>[2x]MPINRPNLNLNIPPLNIVAAYDGAEIPSTNKHLKNNFNSLHNQMRKMPVSHFKEALDVPDYSGMRQSGFFAMSQGFQLNNHGYDVFIHARRESPQSQGKFAGDKFHISVLRDMV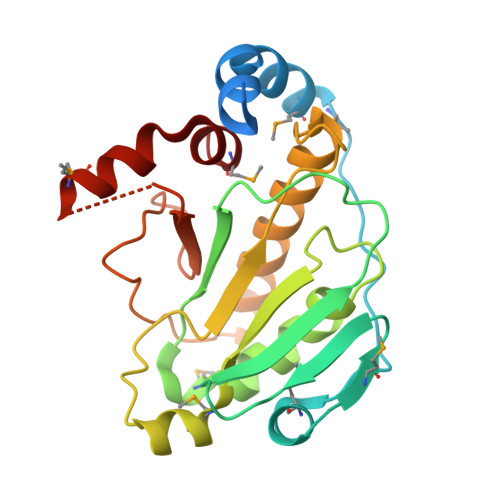PQAFQALSGLLFSEDSPVDKWKVTDMEKVVQQARVSLGAQFTLYIKPDQENSQYSASFLHKTRQFIECLESRLSENGVISGQCPESDVHPENWKYLSYRNELRSGRDGGEMQRQALREEPFYRLMTE2-PHOSPHOGLYCERIC ACID 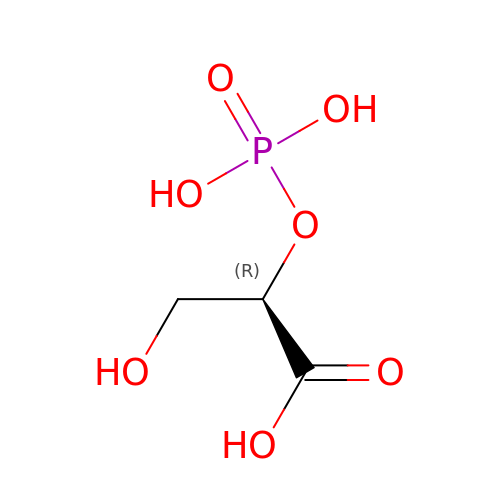| C3 H7 O7 P | GXIURPTVHJPJLF-UWTATZPHSA-N> MEEYRVEMLNKAADGRVMAFEPAVIRAQPGDTVTFVAKDKGHNSALMKGGAPEGAETWKGKINEEITVTLSKPGVYMYQCAPHVGMGMIGAIVVGEPANLEAVKGIKYPGKSKAAA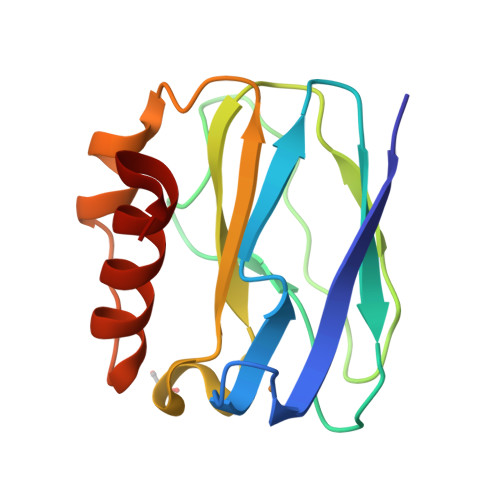EKIFAEIESGG The lysosomal enzyme β-galactocerebrosidase (GALC, also known as β-galactosylceramidase; glycosyl hydrolase family 59) is essential for the normal catabolism and recycling of galactosphingolipids. GALC catalyzes the removal of the terminal galactose moiety from substrates including galactosylceramide, the principal lipid component of myelin, and psychosine, a cytotoxic metabolite. Krabbe disease (also known as globoid cell leukodystrophy) is a rare, inherited autosomal recessive disorder caused by loss of GALC function, leading to devastating and ultimately fatal neurodegeneration. Removal of the galactosyl moieties by GALC occurs via a retaining two-step glycosidic bond hydrolysis reaction.

Of the aza/iminosugars tested, DGJ and nortropane DGN are the weakest inhibitors. Only lactam IGL and DGJ possess a functional group on the ring corresponding to C2 of the substrate and in both these structures this group is able to form additional hydrogen bonds with N181 and E258. Despite these additional interactions DGJ and IGL do not confer greater global stabilization than pyrrolidine DIL. 3 twisted-boat conformation allows DGJ to form a hydrogen bond with the nucleophile E258. 3 twisted-boat conformation is favoured by 14 kcal mol–1 over the chair conformation for DGJ. Due to the position of the nitrogen in DGJ and the orientation of DIL in the active site neither of these molecules can form direct hydrogen bonds with E182 in the active site. Our data also identifies that it is not only charge but also the position of this charge in the active site that is crucial for stabilization of GALC. Both pyrrolidine DIL and DGJ possess a positive charge on the heterocyclic nitrogen at pH 4.6 but neither of these molecules confers equivalent stabilization as IGF and AGF. Thus position of the ring nitrogen directly adjacent to the negatively charged catalytic residues is critically important for achieving the tightest binding, and the maximum possible stabilization effect.

> HHHHHHIEGRGAYVLDDSDGLGREFDGIGAVSGGGATSRLLVNYPEPYRSEILDYLFKPNFGASLHILKVEIGGDGQTTDGTEPSHMHYELDENYFRGYEWWLMKEAKKRNPDIILMGLPWSFPGWLGKGFSWPYVNLQLTAYYVVRWILGAKHYHDLDIDYIGIWNERPFDANYIKELRKMLDYQGLQRVRIIASDNLWEPISSSLLLDQELWKVVDVIGAHYPGTYTVWNAKMSGKKLWSSEDFSTINSNVGAGCWSRILNQNYINGNMTSTIAWNLVASYYEELPYGRSGLMTAQEPWSGHYVVASPIWVSAHTTQFTQPGWYYLKTVGHLEKGGSYVALTDGLGNLTIIIETMSHQHSMCIRPYLPYYNVSHQLATFTLKGSLREIQELQVWYTKLGTPQQRLHFKQLDTLWLLDGSGSFTLELEEDEIFTLTTLTTGRKGSYPPPPSSKPFPTNYKDDFNVEYPLFSEAPNFADQTGVFEYYMNNEDREHRFTLRQVLNQRPITWAADASSTISVIGDHHWTNMTVQCDVYIETPRSGGVFIAGRVNKGGILIRSATGVFFWIFANGSYRVTADLGGWITYASGHADVTAKRWYTLTLGIKGYFAFGMLNGTILWKNVRVKYPGHGWAAIGTHTFEFAQFDNFRVEAAR>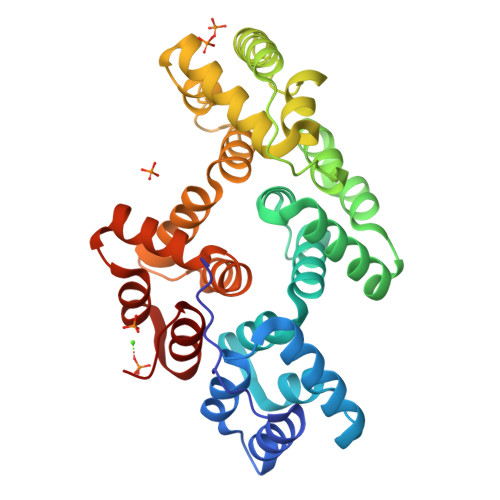 HHATLTVPTTVPSVSEDCEQLRKAFSGWGTNEGLIIDILGHRNAEQRNLIRKTYAETYGEDLLKALDKELSNDFERLVLLWALDPAERDALLANEATKRWTSSNQVLMEIACTRSANQLLHARQAYHARYKKSLEEDVAHHTTGDFHKLLLPLVSSYRYEGEEVNMTLAKTEAKLLHEKISNKAYSDDDVIRVLATRSKAQINATLNHYKNEYGNDINKDLKADPKDEFLALLRSTVKCLVYPEKYFEKVLRLAINRRGTDEGALTRVVCTRAEVDLKVIADEYQRRNSVPLTRAIVKDTHGDYEKLLLVLAGHVEN> GLGKGGAK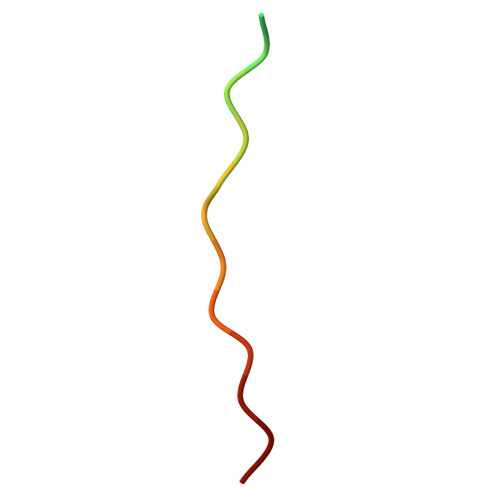RHRKVLRDN>GSHMGTPKPRILPWLVSQLDLGQLEGVAWVNKSRTRFRIPWKHGLRQDAQQEDFGIFQAWAEATGAYVPGRDKPDLPTWKRNFRSALNRKEGLRLAEDRSK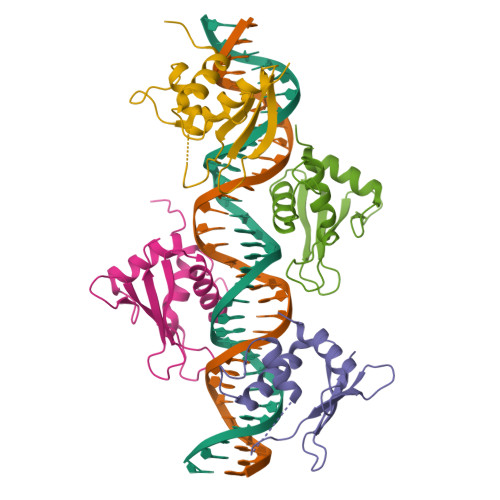DPHDPHKIYEFVNSG[4x]>[2x]GSPAQLDPFYTQGDSLTSEDHLDDSWVTVFGFPQ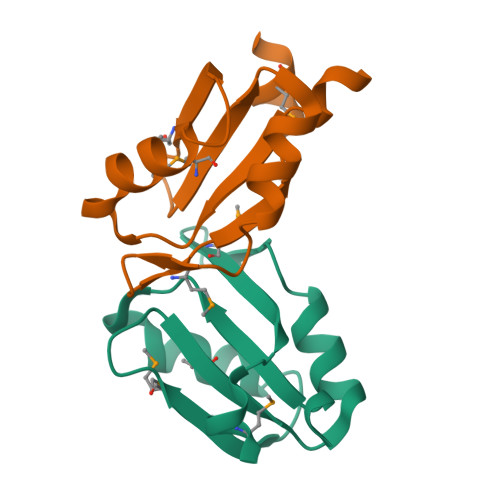ASASYILLQFAQYGNILKHVMSNTGNWMHIRYQSKLQARKALSKDGRIFGESIMIGVKPCIDKSVMESSDRCALSSPSLAFTP> GPASSNLIKQLQERGLVAQVTDEEALAERLAQGPIALYCGFDPTADSLHAGHLVPLLCLKRFQQAGHKPVALVGGATGLIGDPSFKAAERKLNTEETVQEWVDKIRKQVAPFLDFDCGENSAIAANNYDWFGNMNVLTFLRDIGKHFSVNQMINKEAVKQRLNREDQGISFTEFSYNLLQGYDFACLNKQYGVVLQIGGSDQWGNITSGIDLTRRLHQNQVFGLTVPLITKADGTKAGKTEGGAVWLDPKKTSPYKFYQFAINAADADVYRWLKFGTFMSIEEINALEEEDKNSGKA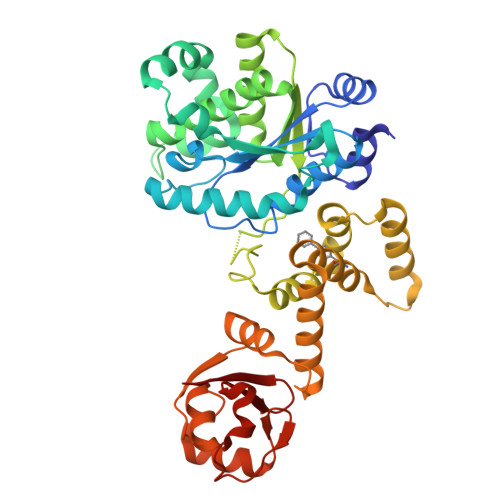PRAQYVFAEQVTRLVHGEEGLQAAKRITECLFSGSLSALSEADFEQLAQDGVPMVEMEKGADLMQALVDSELQPSRGQARKTIASNAITINGEKQSDPEYFFKEEDRLFGRFTLLRRGKKNYCLICWK> MASRADKASSIELKFDRNKGEVGDILIGTVRINNIKNFAGFQVNIVYDPKVLMAVDPETGKEFTSSTFPPGRTVLKNNAYGPIQIADNDPEKGILNFALAYSYIAGYKETGVTEESGIIAKIGFKILQKKSTAVKFQDTLSMPGAILGTQLFDWDGEVITGYEVIQPDVLSLGDEPYEVEHHHHHH;> MNNDSTDKTTVSGYISVDFDYPPESESKIKSGFNVKVAGTELSTKTDEKGYFEISGIPGDMREFTLEISKRNYLKRNVTVNGTGKLVVSTEDNPLILWAGDVERKGVQDNAINMVDVMEISKVFGTRAGDEEYVAELDLNMDGAINLFDIAIVIRHFNALPSRY

In addition, cellulosomes are central elements for the production of readily available sugars in the gastrointestinal tract of a variety of mammals4. It is now well established that a wide array of highly ordered protein-protein interactions involving dockerin and cohesin modules (defined herein as Doc and Coh, respectively) mediate both cellulosome assembly and cellulosome cell-surface attachment. Primary scaffoldins, in addition to containing multiple type-I Cohs, have a divergent type-II Doc that binds to type-II Cohs located in cell-surface anchoring scaffoldins, providing a mechanism to tether the cellulosome to the bacterial cell envelope. In addition to ScaA, inspection of C. thermocellum genome revealed the presence of an ORF (Cthe_1806) encoding a protein comprising 2177 amino acids and containing a putative type-II Doc, which was termed CipB. Type-II Docs of primary scaffoldins ScaA and CipB in C. thermocellum possess two distinct Coh-binding surfaces that recognize different Coh partners.

Thus, in order to probe the mechanism by which CipB XDoc binds to ScaF and ScaA XDoc recognises ScaC2, the crystal structures of ScaF XDoc in complex with ScaC2 Coh (CtCohScaC2-XDocScaA) and CipB XDoc bound to ScaF (CtCohScaF-XDocCipB) were solved. Strikingly, the data revealed that the two Docs bound ScaF and ScaC2 in different orientations. Thus, ScaA (helix 3) and CipB (helix 1) XDocs bound ScaF Coh in opposite orientations. The binding site for ScaF is located primarily in helix 3 of ScaA XDoc and helix 1 of CipB XDoc and is more polar. When CtCohScaF-XDocScaA and CtCohScaF-XDocCipB complexes were overlaid a high structural similarity between the Doc and Coh structures was observed (0.6 Å for 166 Cα atoms of the Coh alone and 1.0 Å for 55 Cα atoms of the Doc module). Doc residues that bind ScaF Coh were highly conserved with the exception of Val115 and Ser121 from CipB XDoc, which correspond to Gln145 and His151, respectively, in ScaA XDoc. ScaA XDoc makes two extra hydrogen bonds with the ScaF Coh through Asn122 and His151, which are compensated in the CipB XDoc-ScaF Coh complex by extra polar contacts established between the side chain of Arg104 of CipBXDoc with Gly166 of ScaF Coh. Inspection of the Coh-Doc interface when ScaF is the Coh partner reveals a much more extensive hydrogen-bonding network when compared to the complexes involving ScaC2 Coh. Binding to ScaF Coh involves the establishment of very important polar contacts between the side chains of Asn158/Asn122 with the Coh. To summarize, the structural and biochemical data here show that the ScaA and CipB XDoc modules bind to ScaC2 and ScaF Cohs in opposite orientations, and different helices thus dominate recognition of the different Cohs.>[2x]MKPKVVLTHWVHPEIIELLSASADVIPNTTRETLPRSEVIARAK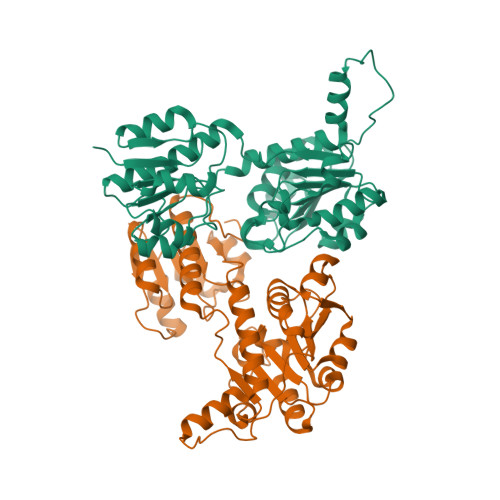DADALMAFMPDSIDSAFLEECPKLRVIGAALKGYDNFDVNACTRHGVWLTIVPDLLTIPTAELTIGLLLGLTRHMLEGDRQIRSGHFQGWRPTLYGSGLTGKTLGIRGMGAVGRAIAQRLAGFEMNLLYCDEIPLNAEQEKAWHVQRVTLDELLEKCDYVVPMVPMAAETLHLIDATALAKMKTGSYLINACRGSVVDENAVIAALASGKLAGYAADVFEMEEWIRADRPQAIPKALLDNTAQTFFTPHLGSAVKEVRLEIERQAAMNIIQALAGEKPMGAINQPYPGVKAALE>MFVDQVKVYVKGGDGGNGMVAFRREKYVPKGGPAGGDGGKGGDVVFEVDEGLRTLMDFRYKKHFKAIRGEHGMSKNQHGRNADDMVIKVPPGTVVTDDDTKQVIADLTEHGQRAVIARGGRGGRGNSRFATPANPAPQLSENGEPGKERYIVLELKVLADVGLVGFPSVGKSTLLSVVSSAKPKIADYHFTTLVPNLGMVETDDGRSFVMADLPGLIEGAHQGVGLGHQFLRHIERTRVIVHVIDMSGLEGRDPYDDYLTINQELSEYNLRLTERPQIIVANKMDMPEAAENLEAFKEKLTDDYPVFPISAVTRE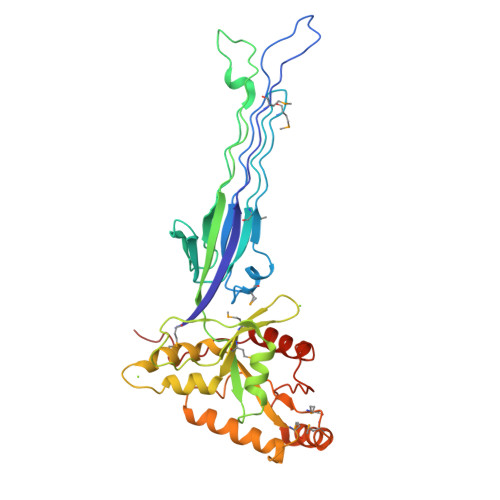GLRELLFEVANQLENTPEFPLYDEEEL[2x]> MFQQLSARLQEAIGRLRGRGRITEEDLKATLREIRRALMDADVNLEVTRDFVERVREEALGKQVLESLTPAEVILATVYEALKEALGGEARLPVLKDRNLWFLVGLQGSGKTTTAAKLALYYKGKGRRPLLVAADTQRPAAREQLRLLGEKVGVPVLEVMDGESPESIRRRVEEKARLEARDLILVDTAGRLQIDEPLMGELARLKEVLGPDEVLLVLDAMTGQEALSVARAFD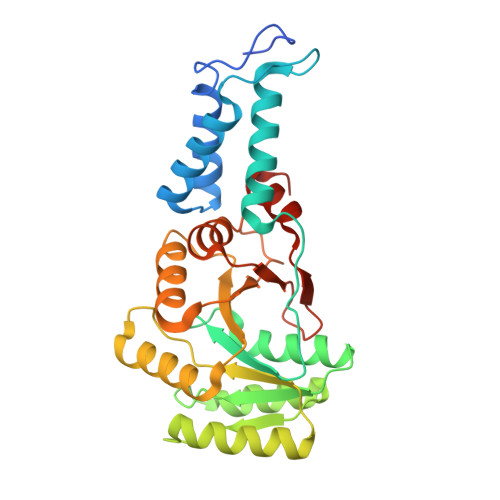EKVGVTGLVLTKLDGDARGGAALSARHVTGKPIYFAGVSEKPEGLEPFYPERLAGRILGMGDVASL> MGVSYEEFQVLVRRVDRME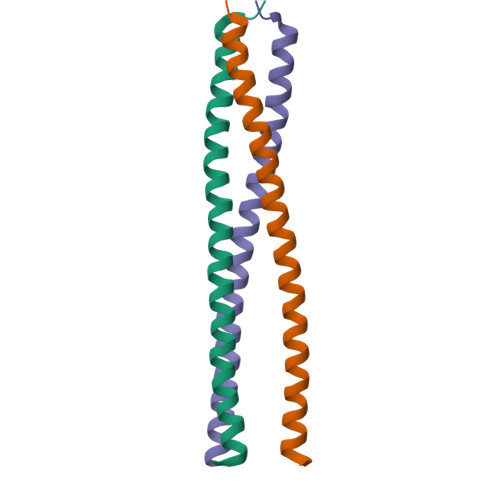HSIGSIVSKIDAVIVKLEIMERAKLKRREVLGRLLDGVAEDERLG> VVGGTEAQRNSWPSQISLQYRSGSSWAHTCGGTLIRQNWVMTAAHCVDRELTFRVVVGEHNLNQNNGTEQYVGVQKIVVHPYWNTDDVAAGYDIALLRLAQSVTLNSYVQLGVLPRAGTILRNNSPCYITGWGLTRTNGQLAQTLQQAYLPTVDYAICSSSSYWGSTVKNSMVCAGGDGVRSGCQGDSGGPLHCLVNGQYAVHGVTSFVSRLGCNVTRKPTVFTRV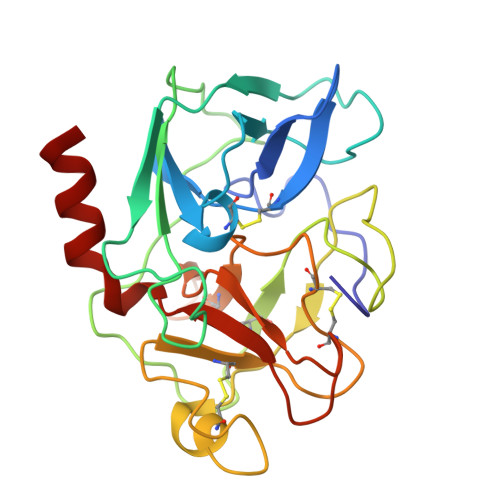SAYISWINNVIASN> GSHMSNITYVKGNILKPKSYARILIHSCNCNGAWGGGIAYQLALRYPKAEKDYVEVCEKYGSNLLGKCILLPSYENSDLLICCLFTSSFGGSSHGEKQSILNYTKLALDKLKTFREAKDK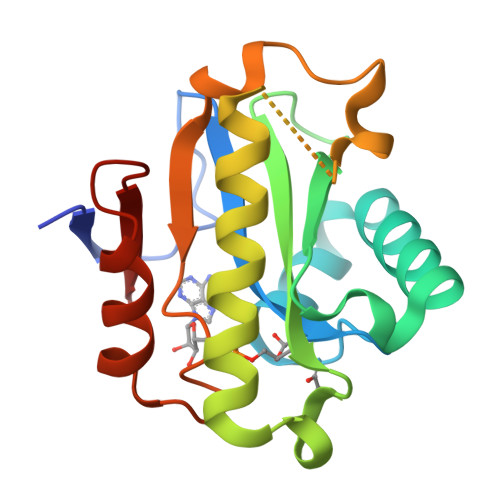TRTSEDSIGDYLNGHIKYPIGEYKLEMPQINSGIFGVPWKETERVLEEFSGDMSFTVYQL>[4x]MAHHHHHHMVKVGINGFGRIGRLVFRASLERTDVEVVAINDIMMTPDYMIYMIKYDSVHGKFNGKLEYTENSIKVNGREIHVFCEREPEKLPWGQYGVEYVVESTGVFTKLDTASKHLKGGAKRVVISAPADTPTFVMGVNNHEFKPEMTVINNASCTTNCLAPIAAVLHENFGIVEGLMTTVHALTATQPTVDAPSKKD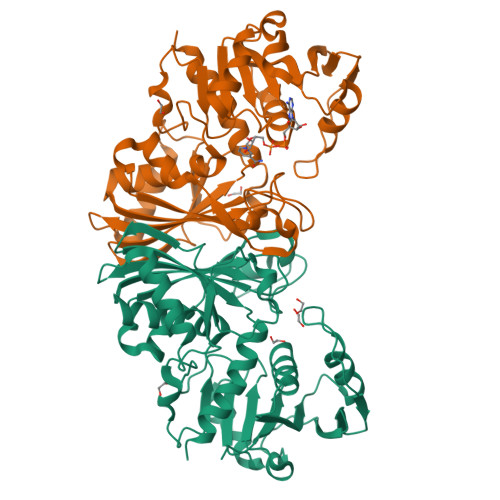WRGGRAAGYNIIPSSTGAAKAVGLVIPSLNGKLTGMAFRVPTADVSVVDLTCRLEKPATKKQIDEAMKKASESERFKGILKYTEEEVVSSDFIHDSASSTYDSKASISLNDHFVKVVAWYDNEWGYSNRVLDLIISTSKVQ>VPSYDSFDSEDYPAALPNHKPKGTFKDYVRDRADLNKDKPVIPAAALAGYTGSGPIQLWQFLLELLTDKSCQSFISWTGDGWEFKLSDPDEVARRWGKRKNKPKMNYEKLSRGLRYYYDKNIIHKTAGKRYVYRFVCDLQSLLGYTPEELHAMLDVK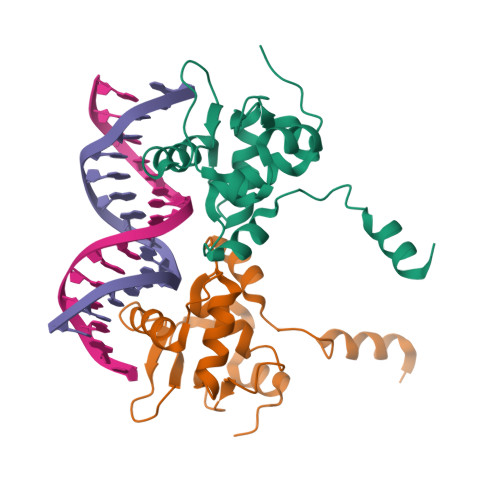PDADE[2x]> MSGSLQADLGKKSLTRLQAESSAAIHATAKWTTENLAKTQAAQAERAKAAMLSQQAAKAKQAKLTQHLKDVVDRALQNNKTRPTVIDLAHQNNQQMAAMAEFIGRQKAIEEAR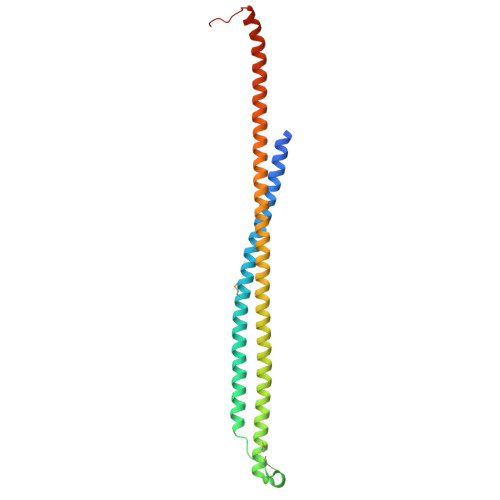KKAEREAKRAEEAYQAALRAQEEEQRKQAEIERKLQEARKQEAAAKAKAEADRIAAEKAEAEARAKAEAERRKAEEARKALFAKAGIKDTPLEHHHHHH Carbon monoxide dehydrogenase (CODH) and acetyl-CoA synthase (ACS) play major roles in the global carbon cycle through the consumption of CO and CO2 gases, production of acetate, and breakdown of acetate for methane generation. By contrast, methanogenic archaea employ four copies of CODH (α2ε2 heterotetramers) and eight copies of ACS (β monomers) that interact stably with eight copies of CFeSP (γδ heterodimers) to form a massive 2.2 MDa complex called the acetyl-CoA decarbonylase/synthase (ACDS) complex. ACDS plays a central role in that process, wherein the A-cluster of ACS cleaves acetyl-CoA into CO and a methyl moiety, the C-cluster of CODH oxidizes CO to CO2, and the corrinoid of CFeSP receives the methyl moiety, which is reduced to methane in downstream methanogenic metabolism. Through plunge freezing of the ACDS complex, we captured multiple subcomplexes including a CODH tetramer, a CODH/ACS pentamer, and a CODH/ACS hexamer and characterized these subcomplexes via cryogenic electron microscopy (cryo-EM).

Using a traditional blot-plunging method, α2ε2 CODH subcomplexes were observed. Sufficient CODH subcomplex was present on the grid to generate a high-resolution reconstruction, however, in 2D and 3D classifications of CODH particles, there were no classes containing additional density consistent with ACS. Here, we observe a similar phenomenon, wherein the full 2.2 MDa ACDS complex is dissociated to a lesser extent on the chameleon than on a blot-plunger; in both the blot-plunged specimen and the chameleon-plunged specimen, CODH particles were observed, but CODH/ACS subcomplexes were only observed in the chameleon-plunged specimen, suggesting that the ACDS complex underwent more dissociation under blot-plunging conditions. The use of two plunging methods allowed us to capture two snapshots of MetCODH, with global resolutions of 2.8 and 3.3 Å for the maps from chameleon and Cp3-plunged samples, respectively. The MetCODH α2ε2 heterotetramer shares the same topology as MebCODH and harbors the same set of metallocofactors, including E- and F-clusters, which are not present in monofunctional and acetogenic CODHs. In the structures of MetCODH without ACS bound, this CO channel is closed. In both cases, helix αA shifts toward helix αB to close the gas channel and block CO release. Additionally, helix αA residue Arg500(Met)/Arg142(Moor) has repositioned so that it no longer hydrogen bonds to the A-cluster coordinating Gly279(Met)/Gly596(Moor). This type of protein motion in CODH is quite interesting, as conformational motion is not precedented in CODHs.

>[2x]MSKLTTGSFSIEDLESVQITINNIVGAAKEAAEKAEEELGPMGPTPFPTAATVRDWSFTLFDRYEPVYTPMCDQCCYCTFGPCNLEGNRRGACGLDMKGQAAREFFLRCITGCACHSAHGRHLLDHIISIFGEDMPINMGASNVIAPNIQLITGRQPKTLGDLKPIMEYVEEELGQLLATVHAGQEGAAIDYDNKAMLAGILDHVGMEVSDIAQVTALGFPKSDPEAPLVEVGMGTLDASKPVIIAIGHNVAGVTYIMDYMEDNNLTDKMEIGGLCCTAFDMTRYKREDRKPPYAKIVGTISKELKVVRSGIPDVIVIDEQCVRADLVEEGKKLKIPVIASNEKVMYGLPDRTNDDVDAIIEDIKTGKIPGCVMLDYEKLGELVPRLAMEMAPLREGISAIPSDEEMASLVAKCVACGECALACPEELDIPDAIQAAKEGDFTALDFLHDLCVGCRRCEQVCNKEIPILSVIDKAAQKAIAEEKGLVRAGRGQVSDAEIRAEGLNLVMGTTPGVIAIIGCANYPAGSKDVYRIAEEFLNRNYIVAVSGCSAMDIGMYKDADGKTLYERFPGRFERGNILNTGSCVSNSHISGTCHKVAAIFAGRNLSGNLAEIADYTLNRVGAVGLAWGAYSQKAAAIGTGCNMYGIPAVLGPHSGKYRRALIAKTYDENKWKVYDSRNGSELDIPPSPEFLITTAETWQEACVLLAKNCIRPSDNNMGRSIKLTHWIELSEKYLGVLPEDWWKFVRHEADLPLSRREELLKKLETEHGWEIDWKKKKIISGPKIKFDVSSQPTNLKRLCKEA;>MVDTTKNTKLFTSYGVKTSKAITTEVAAKLISKAKRPLFVVGTGVLDPELLDRAVKIAKAKNIPIAATGSSMPGFVDKDVNAKYINLHQLGFYLTDPDWPGLDGNGNYDTIILLGHKKYYINQVLSAVKNFSDVKSISIDRNYIQNATMSFGNLSKADHIAALDEVIDLL[2x]5'-O-[(S)-hydroxy{[(S)-hydroxy(phenoxy)phosphoryl]oxy}phosphoryl]thymidine | C16 H20 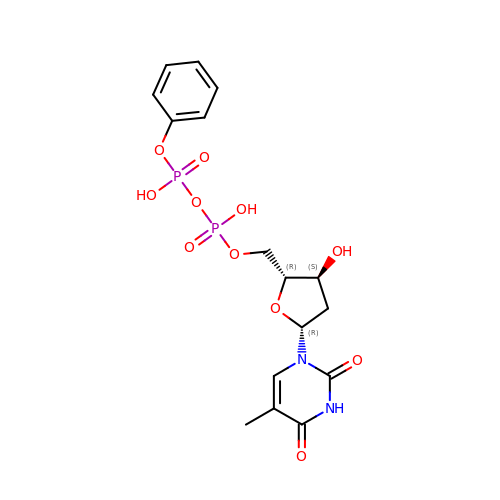N2 O11 P2 | BANJVYKYIQPYKP-BFHYXJOUSA-N> KSH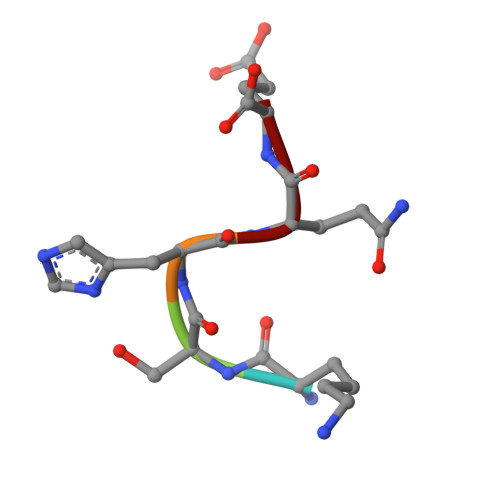QE> SRGLEVSHRLA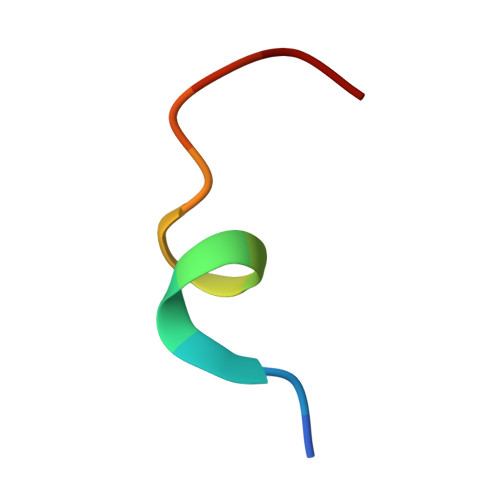PW>[4x]GMDTRKLLLTAQEISRMKGEHKVHFLNPGAVRVNKSLGDAVGLRHMGIHLIQIEPGKESTEYHLHHYEEEAVYVLSG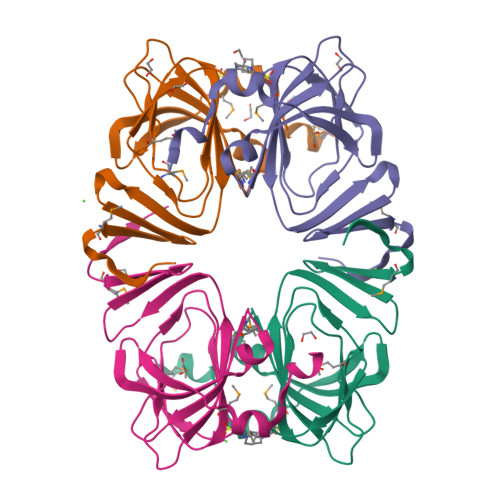KGTLTMENDQYPIAPGDFVGFPCHAAAHSISNDGTETLVCLVIGQRLDQDVVDYPNQHKRLYRNNGEWNLVDMADIRVLREPTQK>GMAQNIYDQPDFFAGYSQLGRSIEGLDGAAEWPAL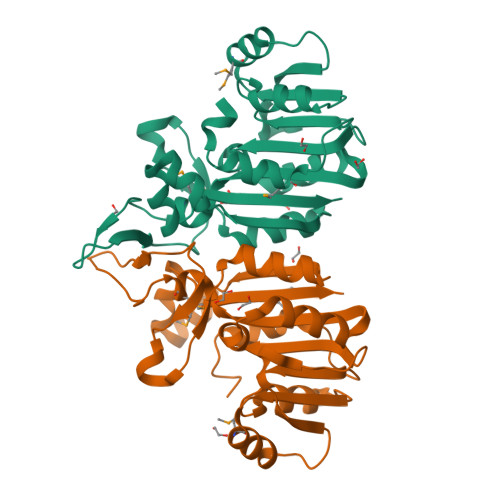RAMLPEVGGLRIVDLGCGFGWFCRWAHEHGASYVLGLDLSEKMLARARAAGPDTGITYERADLDKLHLPQDSFDLAYSSLALHYVEDVARLFRTVHQALSPGGHFVFSTEHPIYMAPARPGWAIDAEGRRTWPIDRYLVEGPRKTDWLAKGVVKHHRTVGTTLNALIRSGFAIEHVEEFCPTDAQITARPELAEELDRPMFLLVSARR[2x]> MTGIPTVTARPWTQRPRAENSTTNPTYFFTFGDSYSQTGFSASGTQPSASNPMGNPDLGIGTTTNGPNWIGYLTTTENASLVLSYNLAAGGATIDNALVPAYPGDLASQFRLFEDVYADKPASAPWSAEDAVFGVWIGINDIGNAYYSTDAETYTPKLISRLESLVEEVYKNGGRKFLFLNV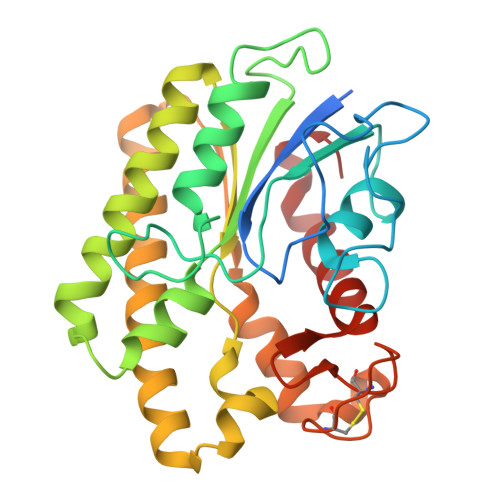PPTSRSPLFLEQGEEVVKQHAEYLSVYNENLEGMVDDFTKKKGDVTTVLYDSWSFMTKILDDPTAYGFPDATCINDDGTSCIWWNNYHPGMKYHLLQAEDMKPKLRKLGGW>GSHMAKTYDYLFKLLLIGDSGVGKTCVLFRFSEDAFNSTFISTIGIDFKIRTIELDGKRIKLQIWDTAGLERFREITTAYYRGAMGIMLVYDITNEKSFDNIRNWIRNIEEHASADVEKMILGNKCDVNDKRQVSKERGEKLALD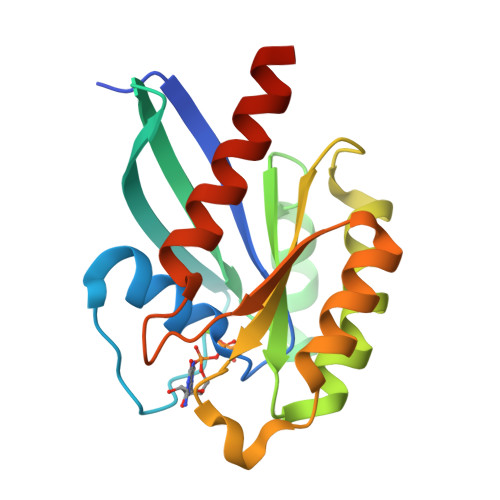YGIKFMETSAKANINVENAFFTLARDIKAKMDKKLEGNS[2x]> GSDELYRQSLEIISRYLREQATGAKDTKPMGRSGATSRKA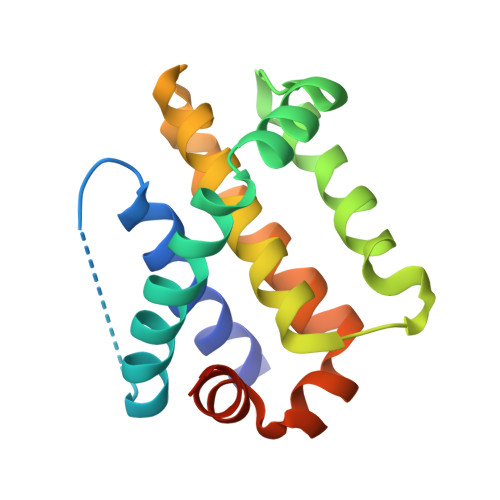LETLRRVGDGVQRNHETAFQGMLRKLDIKNEDDVKSLSRVMIHVFSDGVTNWGRIVTLISFGAFVAKHLKTINQESCIEPLAESITDVLVRTKRDWLVKQRGWDGFVEFFHVEDLEGG> ANFVTDSEVTKLKWSKAPCRFCGTGCGVTVAVKDNKVVATQGDPQAEVNKGLNCVKGYFLSKIMYGQDRLTRPLMRMKNGKYDKNGDFAPVTWDQAFDEMERQFKRVLKEKGPTAVGMFGSGQWTVWEGYAAAKLYKAGFRSNNIDPNARHCMASAAAGFMRTFGMDEPMGCYDDFEAADAFVLWGSNMAEMHPILWTRVTDRRLSHPKTRVVVLSTFTHRCFDLADIGIIFKPQTDLAMLNYIANYIIRNNKVNKDFVNKHTVFKEGVTDIGYGLRPDHPLQKAAKNASDPGAAKVITFDEFAKFVSKYDADYVSKLSAVPKAKLDQLAELYADPNIKVMSLWTMGFNQHTRGTWANNMVYNLHLLTGKIATPGNSPFSLTGQPSACGTAREVGTFSHRLPADMVVTNPKHREEAERIWKLPPGTIPDKPGYDAVLQNRMLKDGKLNAYWVQVNNNMQAAANLMEEGLPGYRNPANFIVVSDAYPTVTALAADLVLPSAMWVEKEGAYGNAERRTQFWHQLVDAPGEARSDLWQLVEFAKRFKVEEVWPPELIAKKPEYKGKTLYDVLYRNGQVDKFPLKDVNAEYHNAEAKAFGFYLQKGLFEEYATFGRGHGHDLAPFDAYHEARGLRWPVVNGKETRWRYREGSDPYVKAGTGFQFYGNPDGKAVIFALPYEPPAESPDKEYPYWLVTGRVLEHWHSGSMTRRVPELYRSFPNAVVFMHPEDAKALGLRRGVEVEVVSRRGRMRSRIETRGRDAPPRGLVFVPWFDASQLINKVTLDATCPISLQTDFKKCAVKIVKV;> QGLVDAMRGPTAIANEPRAPLLYPTENKDIRRTRNYTMQPPTIPHKIDGYQLDKDFNRCMFCHART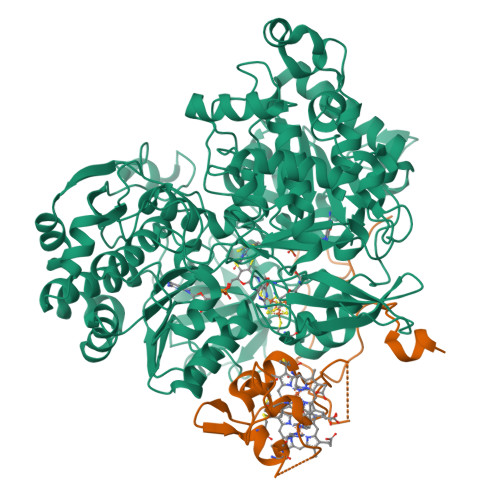RTEETQAIPVSITHYMDRDNNVLADVSPRRYFCTQCHVPQADTKPLIGNNFVDVDTILKRRPGAKGAAK> GSHMANLDRTDDLVYLNVMELVRAVLELKNELSQLPPEGYVVVVKNVGLTLRKLIGSVDDLLPSLPSSSRTEIEGTQKLLNKDLAELINKMRLAQQNAVTSLSEECKRQMLTASHTLAVDAKNLLDAVDQAKVLANLA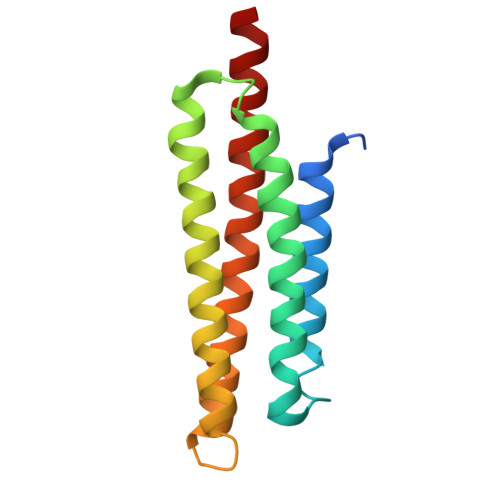H>[40x]ASLTVKAYLLGKEDAAREIRRFSFCCSP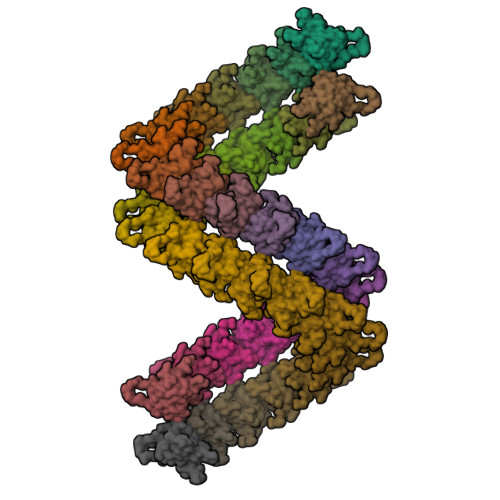EPEAEAEAAAGPGPCERLLSRVAALFPALRPGGFQAHYRDEDGDLVAFSSDEELTMAMSYVKDDIFRIYIKEKKEC> ACYCRIPACIAGEAAYGTCIYQG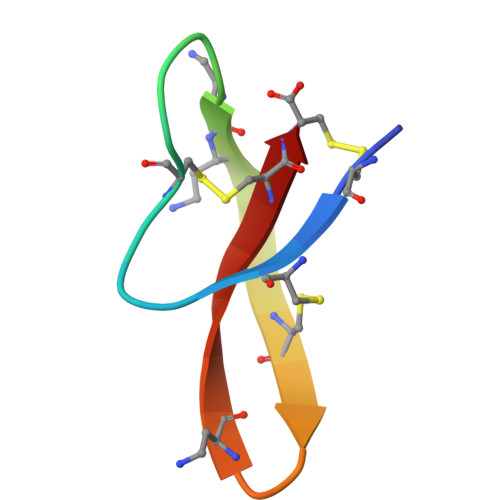ALWAFCC> MSFVKDFKPQALGDTNLFKPIKIGNNELLHRAVIPPLTRMRALHPGNIPNRDWAVEYYTQRAQRPGTMIITEGAFISPQAGGYDNAPGVWSEEQMVEWTKIFNAIHEKKSFVWVQLQVLGWAAFPDNLARDGLRYDSASDNVFMDAEQEAKAKKANNPQHSLTKDEIKQYIKEYVQAAKNSIAAGADGVEIHSANGYLLNQFLDPHSNTRTDEYGGSIENRARFTLEVVDALVEAIGHEKVGLRLSPYGVFNSMSGGAETGIVAQYAYVAGELEKRAKAGKRLAFVHLVEPRVTNPFLT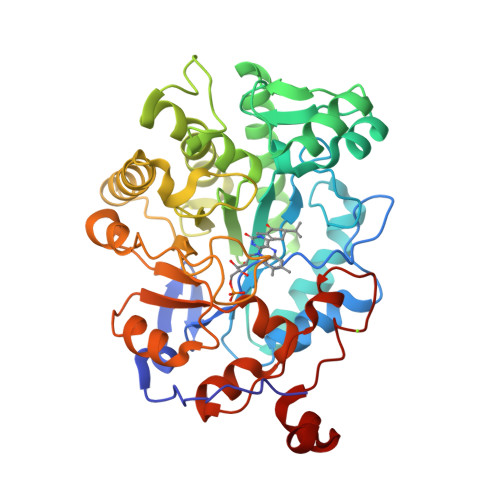EGEGEYEGGSNDFVYSIWKGPVIRAGNFALHPEVVREEVKDKRTLIGYGRFFISNPDLVDRLEKGLPLNKYDRDTFYQMSAHGYIDYPTYEEALKLGWDKK> ISGGDAIYSSTGRCSLGFN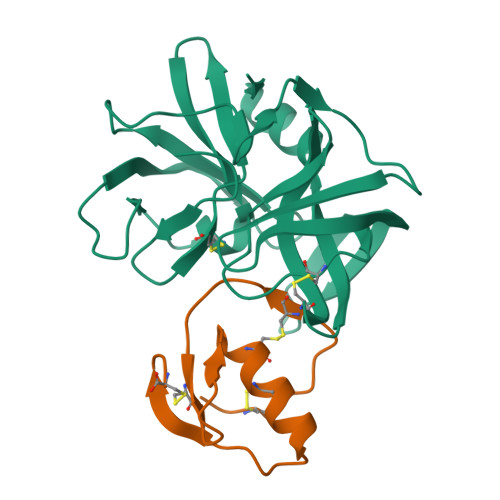VRSGSTYYFLTAGHCTDGATTWWANSARTTVLGTTSGSSFPNNDYGIVRYTNTTIPKDGTVGGQDITSAANATVGMAVTRRGSTTGTHSGSVTALNATVNYGGGDVVYGMIRTNVCAEPGDSGGPLYSGTRAIGLTSGGSGNCSSGGTTFFQPVTEALSAYGVSVY;> VDCSEYPKPACTHEYRPLCGSDNKTYGNKCNFCNAVVESNGTLTLSHFGKC A-1(L) is a Myoviridae cyanophage isolated in 1970s9 that specifically infects the model cyanobacterium Anabaena sp. PCC 7120. Using cryo-electron microscopy (cryo-EM), we solved the structure of A-1(L) tail machine, which consists of three parts: a 205-Å-long neck, a 1045-Å-long contractile tail with a complicated baseplate, and six pairs of tail fibers. The dodecameric gp2 portal, the pentadecameric gp5 and the hexameric gp7 sequentially constitute the neck of A-1(L), to which five neck fibers are attached. The long and contractile tail of A-1(L) contains 24 rings of gp10 hexamers that form the tube, surrounded by the sheath of 24 helically stacked gp9 hexamers.

Besides the baseplate, the 1045-Å-long tail of A-1(L) is composed of one tube initiator/hexameric gp18, one sheath initiator/hexameric gp30, the tube and sheath that consist of helically stacked 24 rings of hexameric gp10 and gp9 in two layers, respectively, surrounding the tape measure protein (TMP) gp13, in addition to one terminator/hexameric gp8, from the distal to proximal of the neck. Encircling the TMP, the tube forms a six-start helix structure with a helical rise of 36.2 Å and a twist of 36.2°. Each tube subunit adopts a conserved structure, containing a β-barrel domain and an α helix, in addition to a β-hairpin that protrudes towards the next ring to mediate the inter-ring interaction, thus extending the tube. Notably, stacking of two rings of the tube is also maintained by the complementary electrostatic potential. Moreover, the sheath also displays a six-start helix structure similar to the tube, with each subunit possessing three globular domains in addition to two folded termini, N-tail and C-tail. The domain II (residues Ala364-Ser460) of one sheath subunit stabilizes the N-tail (residues Met1-Ile27) of one subunit and the C-tail (residues Thr461-Val505) of adjacent subunit in the succeeding ring, enabling the extension of sheath. Meanwhile, the helix α10 of sheath domain II lies on the concave surface of tube β-barrel domain, further stabilizing the interface between the tube and sheath. However, TMP was proposed to adopt a six-fold helical bundle structure in Myoviridae cyanophage Pam3, which is consistent with our observation for the majority of A-1(L) TMP.

>[18x]MTNFLNGVNIGTPGAYAFYQTTQSRPINVEPFRTCYMVGFASNGVNKNVPTRISNLTDFTNVYGTSASTNSVDLFFKNSQGFGNLYFVNVAIPTRYQIVVTAATAGSYSVTVNGVTKAITVVGGATTTTIAADVISAINNDTVLNKEVLATVGGTSSTVVITSKKPTNTTTAAVTGVIFTLTTTTGTSPSVADYVYTINNTFDPALEAGFVIAPEAFSTFTKSDRLSIQVALENLCSAYRYQWAALIDSGAMSEISNTDRAIAEAATYNSVQGHCSYYYPYLINLDDQQVPPSAAVAGMALYRFVIDGFAEPPAGVNFPLKGVKNVAYKVTWEEQNVANPEGVNCILNKENYGIVVWGARTLSADPNIVFISTRIILNIVINTLNRGYDFDIFNSVGGTATVLDNIQRKTNTLLTTLYQAGLFYGQTTSEAFSVLGDASVQVPSLLQQGLVNMFIWVVPSTIIERLIINIKQTAIGDLEATVALDTAALQSSVEEGTATEGTAPVV;>MAVSKRPFSINSFAVNLNIGNFVDARYWSKCSKIEKTYNTGEYSDGQSNIIYTLPGAIKYPEVVLSKAFSPGDEELINRLIAVNSDPIAWVTVFIQPMYRDGYYNVPQGGKIILEFCTVARATPINEIDTIGSNAAMFECALNPSRIRSDGGNINWWSEPAAQVAEF[18x]> KPVWAPHPTDGFQVGNIVDIGPDSLTIEPLNQKGKTFLALINQVFPAEEDSKKDVEDNCSLMYLNEATLLHNIKVRYSKDRIYTYVANILIAVNPYFDIPKIYSSETIKSYQGKSLGTMPPHVFAIADKAFRDMKVLKLSQSIIVSGESGAGKTENTKFVLRYLTESYGTGQDIDDRIVEANPLLEAFGNAKTVRNNNSSRFGKFVEIHFNEKSSVVGGFVSHYLLEKSRICVQGKEERNYHIFYRLCAGASEDIRERLHLSSPDNFRYLNRGCTRYFANKETDKQILQNRKSPEYLKAGSLKDPLLDDHGDFIRMCTAMKKIGLDDEEKLDLFRVVAGVLHLGNIDFEEAGSTSGGCNLKNKSTQALEYCAELLGLDQDDLRVSLTTRVMLTTAGGAKGTVIKVPLKVEQANNARDALAKTVYSHLFDHVVNRVNQCFPFETSSYFIGVLDIAGFEYFEHNSFEQFCINYCNEKLQQFFNERILKEEQELYQKEGLGVNEVHYVDNQDCIDLIEARLVGILDILDEENRLPQPSDQHFTSAVHQKHKDHFRLSIPRKSK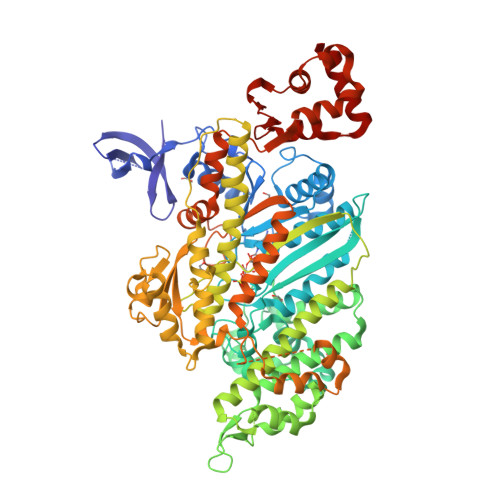LAIHRNIRDDEGFIIRHFAGAVCYETTQFVEKNNDALHMSLESLICESRDKFIRELFESSTNNNKDTKQKAGKLSFISVGNKFKTQLNLLLDKLRSTGASFIRCIKPNLKMTSHHFEGAQILSQLQCSGMVSVLDLMQGGFPSRASFHELYNMYKKYMPDKLARLDPRLFCKALFKALGLNEIDYKFGLTKVFFRPGKFAEFDQIMKSDPDHLAELVKRVNHWL> MSTAVQFRGGTTAQHATFTGAAREITVDTDKNTVVVHDGATAGGFPLARHDLVKTAFIKADKSAVAFTRTGNATASIKAGTIVEVNGKLVQFTADTAITMPALTAGTDYAIYVCDDGTVRADSNFSAPTGYTSTTARKVGGFHYAPGSNAAAQAGGNTTAQINEYSLWDIKFRPAALDPRGMTLVAGAFWADIYLLGVNHLTDGTSKYNVTIADGSASPKKSTKFGGDGSAAYSDGAWYNFAEVMTHHGKRLPNYNEFQALAFGTTEATSSGGTDVPTTGVNGTGATSAWNIFTSKWGVVQASGCLWTWGNEFGGVNGASEYTANTGGRGSVYAQPAAALFGGAWNGTSLSGSRAALWYS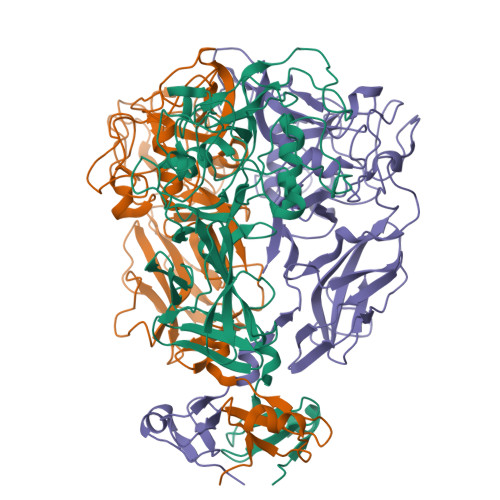GPSFSFAFFGARGVCDHLILE> MEHVAFGSEDIENTLAKMDDGQLDGLAFGAIQLDGDGNILQYNAAEGDITGRDPKQV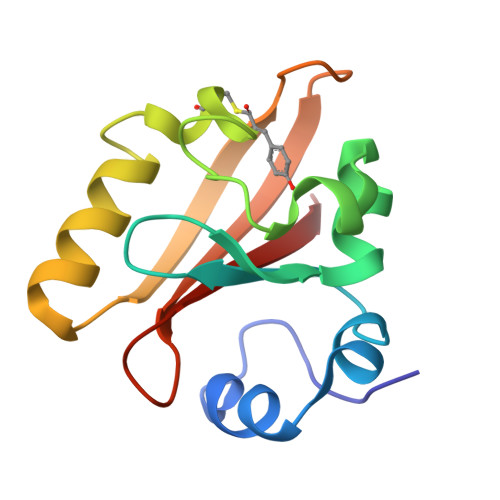IGKNFFKDVAPCTDSPEFYGKFKEGVASGNLNTMFEYTFDYQMTPTKVKVHMKKALSGDSYWVFVKRV> SNVKTENNDHINLK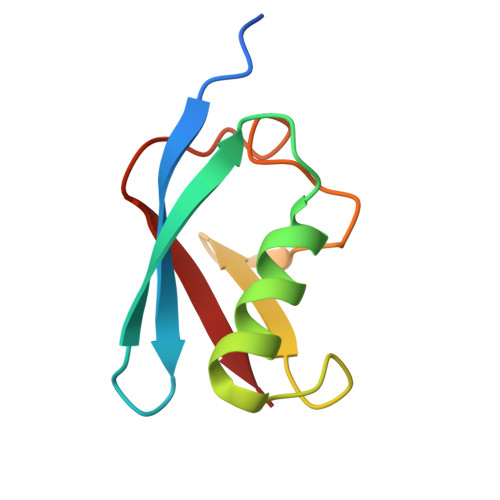VAGQDGSVVQFKIKRHTPLSKLMKAYCERQGLSMRQIRFRFDGQPINETDTPAQLEMEDEDTIDVFQ>MRGSHHHHHHGSMTDTYLHETLVFDNKLSYIDNQRDTDGPAILLLPGWCHDHRVYKYLIQELDADFRVIVPNWRGHGLSPSEVPDFGYQEQVKDALEILDQLGVETFLPVSHSHGGWVLVELLEQAGPERAPRGIIMDWLMWAPKPDFAKSLTLLKDPERWREGTHGLFDVWLDGHDEKRVRHHLLEEMADYGYDCWGRSGRVIEDAYGRNGSPMQMMANLTKTRPIRHIFSQPTEPEYEKINSDFAEQHPWFSYAKLGGPTHFPAIDVPDRAAVHIREFATAIRQGQ[4x]

Arthrobacter nitroguajacolicus Rü61a 1-H-3-hydroxy-4-oxoquinaldine 2,4-dioxygenase (HOD) and Pseudomonas putida 33/1 1-H-3-hydroxy-4-oxoquinoline 2,4-dioxygenase (QDO) were the first dioxygenases discovered to belong to the ABH-fold family. They catalyze the O2-dependent breakdown of N-heteroaromatic quinolone-type substrates with concomitant carbon monoxide production. Atypical for oxygenases, these enzymes promote the activation of the triplet ground-state O2 molecule without the aid of metal centers or external organic co-factors. Kinetic measurements indicate that their reaction mechanism relies on a fast initial step, during which the substrates' 3-hydroxyl group is deprotonated by the His-Asp subset of the triad, thus promoting its activation for molecular oxygen attack (step 1), whilst the nucleophile is not essential.

We next employed xenon pressurization in the crystal state to probe O2 sites experimentally. Electron-rich Xe is quite easily detected by crystallographic methods and has been successfully used to visualize hydrophobic O2 binding sites in proteins. Pressurization of HOD crystals in a quartz capillary at room-temperature under a constant 30 bar Xe atmosphere allowed us to measure X-ray data at 2.9 Å using synchrotron radiation (Table S1†). Fourier difference density maps revealed strong peaks consistent with xenon binding at the B-site (as it overlaps with the substrate's B-ring in the HOD–QND complex) of all four HOD molecules present in the asymmetric unit. Modelling these peaks as water molecules resulted in significant positive residual density post-refinement, supporting the notion that Xe occupies this site (Fig. S5A†). Occupancy refinement of Xe atoms gives values in the 40–60% range. Xe is stabilized at the B-site by the hydrophobic environment of the H102, F136, L140, L143, L156, W160, W185, I192 side chains with the closest atoms 3.8–5.0 Å from the gas atom. Although we performed our experiment at room temperature, which compared to cryo-conditions, allows for enhanced protein, mobility we have not identified additional Xe binding sites in our maps. Overall, experiments and simulations agree that the ABH-fold HOD dioxygenase features an O2 pocket (B-site) within the active site at a location that overlaps with the most hydrophobic portion of its aromatic substrate. Transient O2 storage at the xenon-validated B-site that we have identified overlapping with the hydrophobic portion of the N-heteroaromatic binding site represents a convenient solution to the problem of O2 localization, as one might envisage a mechanism of displacement that upon substrate binding transfers O2 from the B-site to the R-site that is only about 5 Å away, thus organizing both reactants for catalysis.>NSELDRLSKDDRNWVMQTKDYSATHFSRLTEINSHNVKNLKVAWTLSTGTLHGHEGAPLVVDGIMYIHTPFPNNVYAVDLNDTRKMLWQYKPKQNPAARAVACCDVVNRGLAYVPAGEHGPAKIFLNQLDGHIVALNAKTGEEIWKMENSDIAMGSTLTGAPFVVKDKVLVGSAGAELGVRGYVTAYNIKDGKQEWRAYATGPDEDLLLDKDFNKDNPHYGQFGLGLSTWEGDAWKIGGGTNWGWYAYDPKLDMIYYGSGNPAPWNETMRPGDNKWTMTIWGRDADTGRAKFGYQKTPHDEWDYAGVNYMGLSEQEVDGKLTPLLTHPDRNGLVYTLNRETGALVNAFKIDDTVNWVKKVDLKTGLPIRDPEYSTRMDHNAKGICPSAMGYHNQGIESYDPDKKLFFMGVNHICMDWEPFMLPYRAGQFFVGATLNMYPGPKGMLGQVKAMNAVTGKMEWEVPEKFAVWGGTLATAGDLVFYGTLDGFIKARDTRTGELKWQFQLPSGVIGHPITYQHNGKQYIAIYSGVGGWPGVGLVFDLKDPTAGLGAVGAFRELAHYTQMGGSVFVFSL[8x];>YDGTHCKAPGNCWEPKPGYPDKVAGSKYDPKHDPNELNK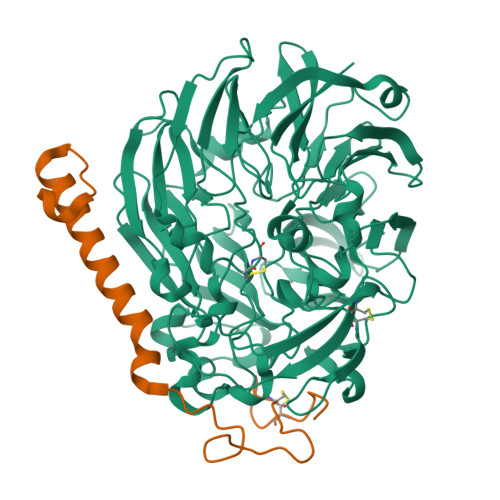QAESIKAMEARNQKRVENYAKTGKFVYKVEDIK[8x]> APMGSDPATACCFSYTARKLPRNFVVDYYETSSLCSQPAVVFQTKRSKQVCADPSESWVQEYVYDLEL

CC chemokine ligands (CCL) comprise 8-14 kDa chemotactic cytokines (chemokines) involved in diverse immune functions. Extensive structural analyses reveal that most chemokines share a common core structure: an N-terminal extension followed by a 310 helical turn, an anti-parallel three-stranded β-sheet, and an α-helix. CC chemokines also readily dimerize, primarily through the formation of an anti-parallel β-sheet at their N-termini. Certain chemokines, e.g. CCL3, CCL4, and CCL5 form polydisperse, high MW reversible polymers in excess of 600 kDa without the assistance of GAG.

The crystal of CCL4 P8A diffracted to 1.6 Å resolution is in space group C2. Unlike our previously reported crystal structure of the wild type CCL4 polymer, the structure of CCL4 P8A is monomeric. CCL4 P8A maintains the typical chemokine fold. However, CCL4 P8A has a distinct structure at the N-terminus. Instead of the extended loop found in wild type CCL4, the absence of proline at position 8 of CCL4 allows aa 6-9 to form a type 1 β-turn so that the N terminus turns back toward the three-stranded β-sheet of CCL4. This permits favorable hydrogen bonds to form between the main chains of residues at the N-terminal loop of CCL4 (Met3 with Cys11; Asp6 with Ala10). All prolines (Pro 7 and 8 in wild type and Pro 7 in P8A mutant) are in the trans configuration, thus the formation of type 1 β-turn is not due to the switch of cis-trans peptidyl bonds of proline. The N-terminal conformation of CCL4 P8A would lead to steric clashes between two monomers of CCL4 P8A, which prevents dimerization, explaining why CCL4 P8A is polymerization deficient. Furthermore, the structure of CCL4 P8A reveals that the P8A mutation promotes the formation of an N-terminal type I β-turn, which prevents the formation of anti-parallel β-sheet essential for CCL4 dimerization. A P8A mutation renders CCL4 predominantly monomeric without disturbing the integrity of its core structure (aa 10-69).>GPKYTMFHYLRAQEFEHGKSRIALTNSVNEALLNPSRVYTFFSSDYVKKVNKATEAAMFLGWVEQLVYDFTDETSEVSTTDKIADITIIIPYIGPALNIGNMLYKDDFVGALIFSGAVILLEFIPEIAIPVLGTFALVSYIANKVLTVQTIDNALSKRNEKWDEVYKYIVTNWLAKVNTQIDLIRKKMKEALENQAEATKAIINYQYNQYTEEEKNNINFNIDDLSSKLNESINKAMININKFLNQCSVSYLMNSMIPYGVKRLEDFDASL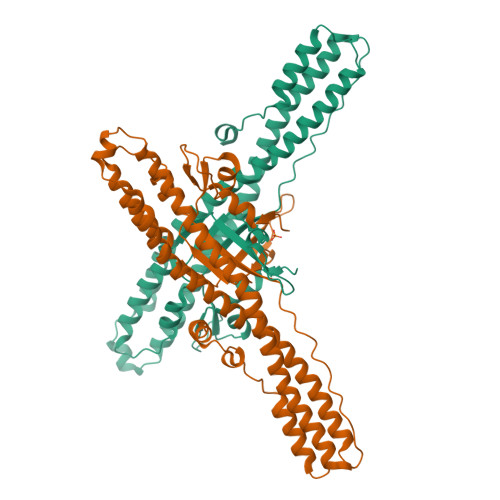KDALLKYIYDNRGTLIGQVDRLKDKVNNTLSTDIPFQLSKYVDNQRLLSTFTEYIK[2x]> GPPGGVTEGIIARVADTVGSGPVNSESIPALTAAETGHTSQVVPSDTMQTRHVKNYHSRSESTVENFLCRSACVFYTTYKNHDSDGDNFAYWVINARQVAQLRRKLEMFTYARFDLELTFVITSTQEQSTTQGQDTPVLTHQIMYVPPGGPVPTKVNSYSWQTSTNPSVFWTEGNAPPRMSIPFIGIGNAYSMFYDGWARFDKQGTYGISTLNSMGTLYMRHVNGGGPGPIVSTVRIYFKPKHVKTWVPRPPRLCQYKKAGNVNFIPTSVTEGRTDITTMKTT;> SPSAEECGYSDRVRSITLGNSTITTQECANVVVGYGVWPAYLKDEEATAEDQPTQPDVATCRFYTLESVMWQQGSPGWWWKFPDALSNMGLFGQNMQYHYLGRAGYTIHVQCNASKFHQGCLLVVCVPEAEMGCATLANKPDPKSLSKGEIASTFESQNSTGETAVQANVINAGMGVGVGNLTIFPHQWINLRTNNSATIVMPYINSVPMDNMFRHNNFTLMVIPFAPLSYSAGATTYVPITVTVAPMCAEYNGLRLAGKQ;> GLPTLATPGSNQFLTSDDFQSPSAMPQFDVTPEMDIPGQVNNLMEIAEVDSVVPVNNTEGKEMSIEAYQIPVQSNPTNGSQVFGFPLTPGASSVLNRTLLGEILNY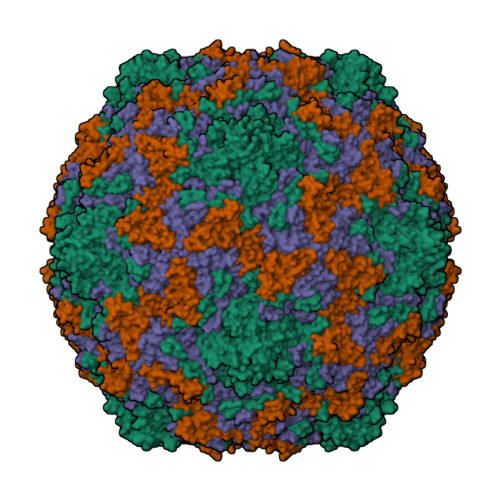YAHWSGSIKLTFMFCGSAMATGKFLLAYSPPGAGAPTTRKEAMLGTHVIWDVGLQSSCVLCIPWISQTHYRYVVMDEYTAGGYITCWYQTNIVVPADAQSDCKILCFVSACNDFSVRMLKDTPFIKQDNFFQ;> GAQVSTQKTGAHETSLNAAGNSVIHYTNINYYKDAASNSANRQDFTQDPGKFTEPVKDIMVKSMPALN4-[(6-fluoropyridin-2-yl)sulfamoyl]benzene-1-sulfonic 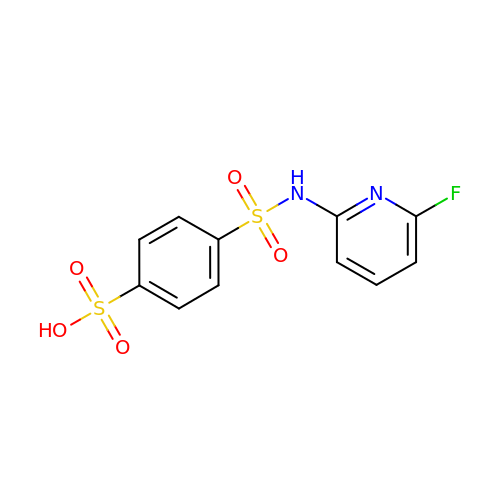acid | C11 H9 F N2 O5 S2 | FAPGWCMQIRKSPW-UHFFFAOYSA-N> MERYENLFAQLNDRREGAFVPFVTLGDPGIEQSLKIIDTLIDAGADALELGVPFSDPLANGPTIQNANLRAFAAGVTPAQCFEMLALIREKHPTIPIGLLMYANLVFNNGIDAFYARCEQVGVDSVLVADVPVEESAPFRQAALRHNIAPIFICPPNADDDLLRQVASYGRGYTYLLSRSGVTGAENRGALPLHHLIEKLKEYHAAPALQGFGISSPEQVSAAVRAGAAGAISGSAIVKIIEKNLASPKQMLAELRSFVSAMKAASRA;> MTTLLNPYFGEFGGMYVPQILMPALNQLEEAFVRAQKDPEFQAQFADLLKNYAGRPTALTKCQNITAGTRTTLYLKREDLLHGGAHKTNQVLGQALLAKRMGKSEIIAETGAGQHGVASALASALLGLKCRIYMGAKDVERQSPNVFRMRLMGAEVIPVHSGSATLKDACNEALRDWSGSYETAHYMLGTAAGPHPYPTIVREFQRMIGEETKAQILDKEGRLPDAVIAC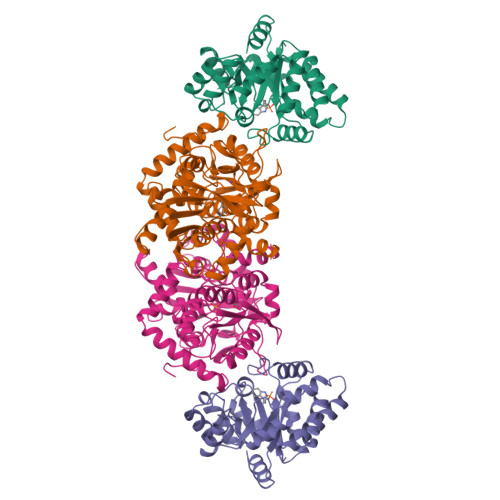VGGGSNAIGMFADFINDTSVGLIGVEPGGHGIETGEHGAPLKHGRVGIYFGMKAPMMQTADGQIEESYSISAGLDFPSVGPQHAYLNSIGRADYVSITDDEALEAFKTLCRHEGIIPALESSHALAHALKMMREQPEKEQLLVVNLSGRGDKDIFTVHDILKARGLI>[2x]MRSRRVDVMDVMNRLILAMDLMNRDDALRVTGEVREYIDTVKIGYPLVLSEGMDIIAEFRKRFGCRIIADFKVADIPETNEKICRATFKAGADAIIVHGFPGADSVRA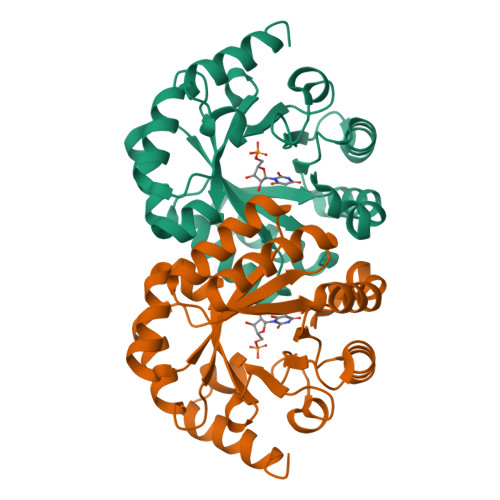CLNVAEEMGREVFLLTEMSHPGAEMFIQGAADEIARMGVDLGVKNYVGPSTRPERLSRLREIIGQDSFLISPGVGAQGGDPGETLRFADAIIVGRSIYLADNPAAAAAGIIESIKDLLNP>[2x]LAAAPVMVNDCTGKVGQAVAEAAVAAGLRLVPLS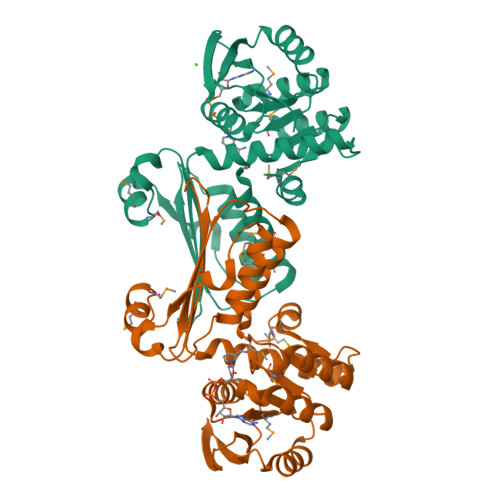LTGPGRGGKRVVIGNVEVDVREVSEREDVVKEVITEYPNVIVVDYTLPAAVNDNAEFYCKQGLPFVMGTTGGDREKLLDVARKSGTYSIIAPQMGKQVVAFVAAMEIMAKQFPGAFSGYTLQVTESHQSTKADVSGTALAVISSLRKLGLDFKDEQVELVRDPKEQMTRMGVPEQHLNGHAFHTYKIISPDGTVFFEFKHNVCGRSIYAQGTVDAVLFLSKKIQEKSEKRLYNMIDVLEGGSMR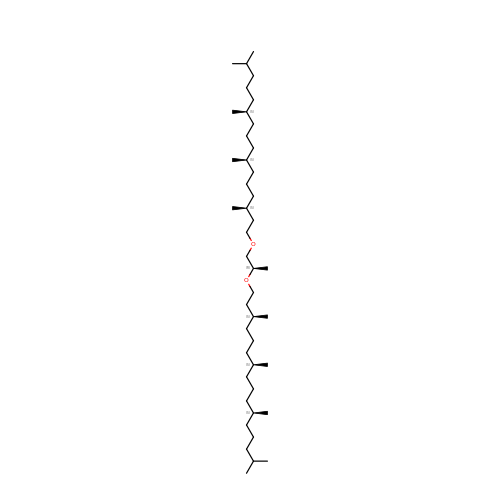1,2-[DI-2,6,10,14-TETRAMETHYL-HEXADECAN-16-OXY]-PROPANE | C43 H88 O2 | ICKFQWWHLUUVMF-FYYCEQFTSA-N N-{2-[2-(1H-imidazol-1-yl)pyrimidin-4-yl]ethyl}-3-(pyridin-3-yl)propan-1-amine 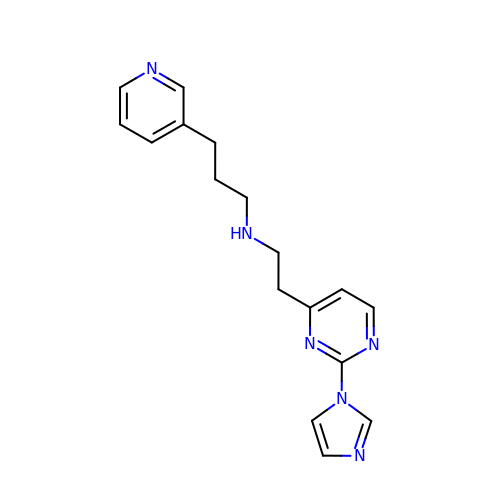| C17 H20 N6 | XOWPXRYZDHLBEA-UHFFFAOYSA-N>[2x]MALKTDIR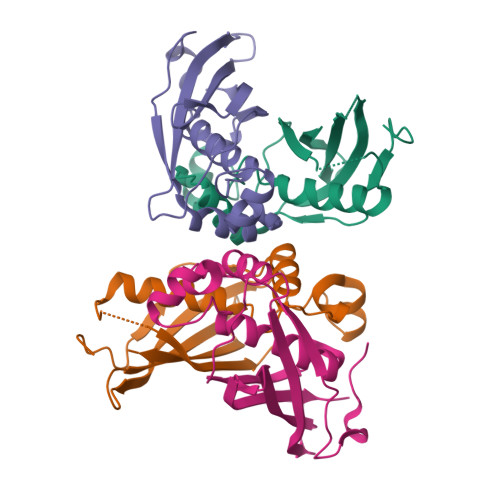GMIWRYPDYFIVGREQCREFARAVKCDHPAFFSEEAAADLGYDALVAPLTFVTILAKYVQLDFFRHVDVGMETMQIVQVDQRFVFHKPVLAGDKLWARMDIHSVDERFGADIVVTRNLCTNDDGELVMEAYTTLMGQQGDGSARLKWDKE;>[2x]MALREFSSVKVGDQLPEKTYPLTRQDLVNYAGVSGDLNPIHWDDEIAKVVGLDTAIAHGMLTMGIGGGYVTSWVGDPGAVTEYNVRFTAVVPVPNDGKGAELVFNGRVKSVDPESKSVTIALTATTGGKKIFGRAIASAKLA> MKFSNITIKNFRNFEKVNINLDNKNVIFGMNDIGKTNFLYALRFLLDKEIRKFGFNKSDYHKHDTSKKIEIILTLDLSNYEKDEDTKKLISVVKGARTSANADVFYIALESKYDDKELYGNIILKWGSELDNLIDIPGRGNINALDNVFKVIYINPLVDLDKLFAQNKKYIFEESQGNESDEGILNNIKSLTDQVNQQIGEMTIIKGFQQEITSEYRSLKKEEVSIELKSEMAIKGFFSDIIPYIKKDGDSNYYPTSGDGRRKMLSYSIYNYLAKKKYEDKIVIYLIEEPEISLHRSMQIALSKQLFEQSTYKYFFLSTH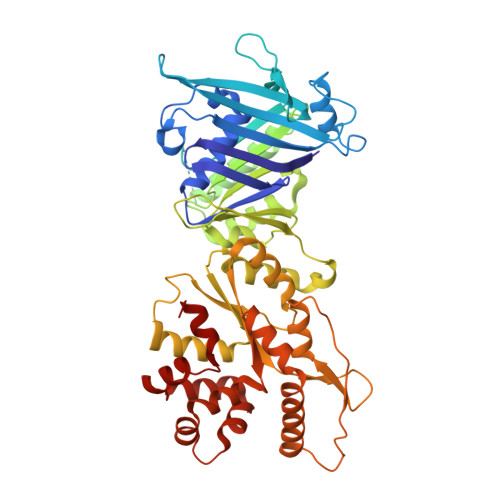SPELLYEMDNTRLIRVHSTEKVVCSSHMYNVEEAYGSVKKKLNKALSSALFAERVLLIEGPSEKILFEKVLDEVEPEYELNGGFLLEVGGTYFNHYVCTLNDLGITHIIKTDNDLKSKKGKKGVYELLGLNRCLNLLGRENLDEITIDIPEDIKGKKKKERLNERKKEIFKQYKNEVGEFLGERIYLSEIDLENDLYSAIGESMKRIFENEDPVHYLQKSKLFNMVELVNNLSTKDCFDVFEHEKFACLKELVGSDRG> DAPEAETQAQETQGQAAARAAAADLAAGQDDEPRILEAPAPDARRVYVNDPAHFAAVTQQFVIDGEAGRVIGMIDGGFLPNPVVADDGSFIAHASTVFSRIARGERTDYVEVFDPVTLLPTADIELPDAPRFLVGTYPWMTSLTPDGKTLLFY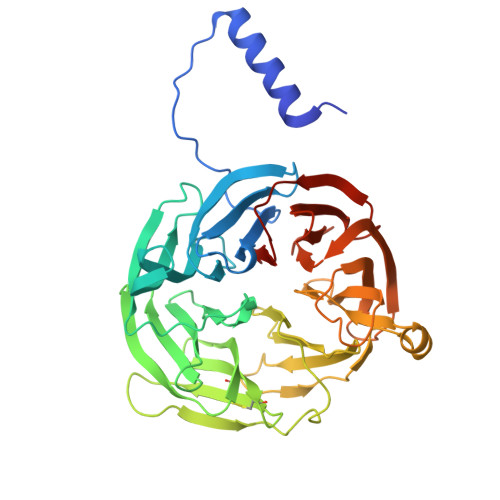QFSPAPAVGVVDLEGKAFKRMLDVPDCYHIFPTAPDTFFMHCRDGSLAKVAFGTEGTPEITHTEVFHPEDEFLINHPAYSQKAGRLVWPTYTGKIHQIDLSSGDAKFLPAVEALTEAERADGWRPGGWQQVAYHRALDRIYLLVDQRDEWRHKTASRFVVVLDAKTGERLAKFEMGHEIDSINVSQDEKPLLYALSTGDKTLYIHDAESGEELRSVNQLGHGPQVITTADMG[({4-[4-(propan-2-yloxy)phenyl]pyridin-2-yl}amino)methanediyl]bis(phosphonic acid) | C15 H20 N2 O7 P2 | 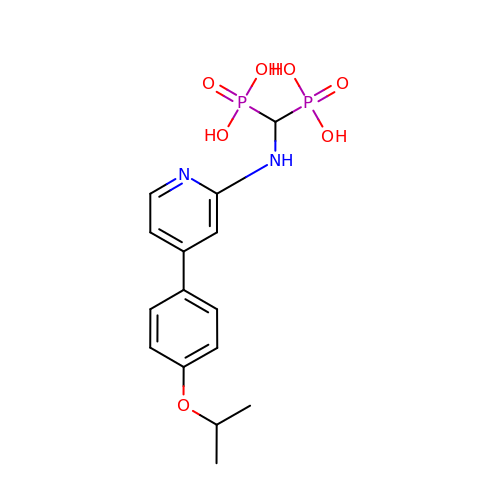DTXBFSJBRGLOHO-UHFFFAOYSA-N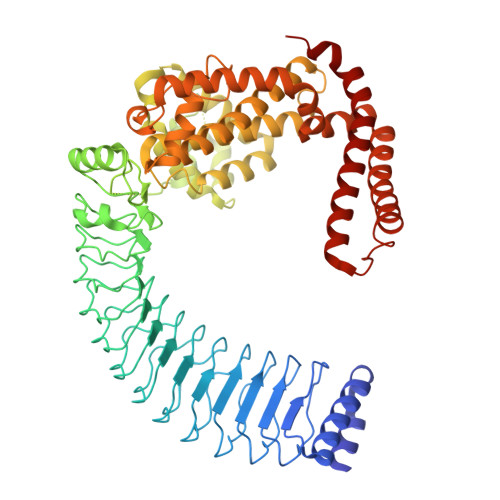> GPVDPAEYDAVWSAWRRAAPAEESRGRAAVVQKMRACLNNGNAVLNVGESGLTTLPDCLPAHITTLVIPDNNLTSLPALPPELRTLEVSGNQLTSLPVLPPGLLELSIFSNPLTHLPALPSGLCKLWIFGNQLTSLPVLPPGLQELSVSDNQLASLPALPSELCKLWAYNNQLTSLPMLPSGLQELSVSDNQLASLPTLPSELYKLWAYNNRLTSLPALPSGLKELIVSGNRLTSLPVLPSELKELMVSGNRLTSLPMLPSGLLSLSVYRNQLTRLPESLIHLSSETTVNLEGNPLSERTLQALREITSAPGYSGPIIRFDMAGASAPRETRALHLAAADWLVPAREGEPAPADRWHMFGQEDNADAFSLFLDRLSETENFIKDAGFKAQISSWLAQLAEDEALRANTFAMATEATSSCEDRVTFFLHQMKNVQLVHNAEKGQYDNDLAALVATGREMFRLGKLEQIAREKVRTLALVDEIEVWLAYQNKLKKSLGLTSVTSEMRFFDVSGVTVTDLQDAELQVKAAEKSEFREWILQWGPLHRVLERKAPERVNALREKQISDYEETYRMLSDTELRPSGLVGNTDAERTIGARAMESAKKTFLDGLRPLVEEMLGSYLNV> MMSILVISGTPRKNGRTRIAASYIRDRFHTDFIDLSESELPLYNGEEEQNE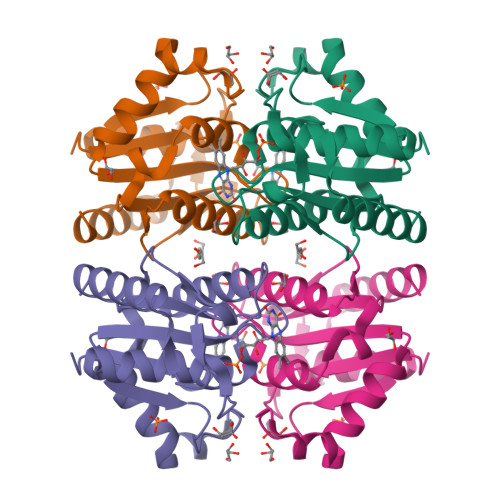LPSVQALRRQVKKSAAVVLLSPEYHSGMSGALKNAIDFLSSDHWAYKPVAIIAAAGGGKGGMNALANMRTVMRGVYANVIPKQLVLDPIHIDMERRTVSEDMAVSLKDMIEELNMFT> MAAVFGIQLVPKLNTSTTRRTFLPLRFDLLLDRLQSTNLHGVLYRALDFNPVDRSATVIQTYPPLNAWSPHHAFIENPLDYRDWTEFIHDRALAFVGVLTQRYPLTQNAQRYTNPLVLGAAFGDFLNARSIDIFLDRLFYDPTQDSPITAITKFPYQWTIDSNVTTDSVRTSAGCKYITLYGYDPSRPSTPATYGKHRPTYATVFYYSTLPARSRLLANLAAGPTVLEHFDSPTYGPHLLLPQTGDVLGYSSSLISQAALLMVESVMDALRDNANASASTAVTRLDQSYHPVTSFDPSTFNTLLQRATNLALLAVQGVQSESAIPAIPTMSDVRSFVARLMAEGDPQQWFPYRVDQILYWPESPFVPPIGPFYAPFRPVNFPFTTGSYTVVPDASRPLRLLPQYRNATITVQQADDAYEDTALSPLITTHGFCVTGGVFTSIYDISGDPTAYPPAQLVDAPNDYFDRERMARRDLFRRLRAPADRSAIKDRAVFDFLASLVNPTTANPVLDTSFSMAYLGASSAHANADEPVILADIRSGSIPGLPIPRRIVQFGYDVVHGSLLDLSRAVPTGTFGLVYADLDQVEDAGTDMPAANRAAIAMLGTALQMTTAGGVSVLKVNFPTRAFWTQVFNLYATHATTLHLVKPTIVNSSEVFLVFGGRQSNGALRSTTALQRALLSLYARNAAIDRAVTHIPFFGVPDDGTSDLGIDAVRLFDPMFSDAVANLPSNALASLVSRVVPSSIMFTRVPSNGPVSTTIYGKRTFLSNRRRARLRDVPMLITTTLVHQRRFTTPPTFTLFSSEAVPVTTLVAAGYNSFISEQTRNPNLAHLLDLGTGPECRILSLIPPTLQVTMSDSRPCAELMASFDPALTAYVQGDYSTAAFWNGIRCDSATAIFTIGAAAAAAGTDLIAFVQQLIPRIVAAGGTRMWLQLNTPLYEVSSLPDLIEIDLRDHVYRFNGGERVEPYADPVPLQQAIAALLPAAALSWHTLSPTCDWLPYIIGVGSPLNLSDINTAISYSRLTPILHIDTTTPPLRVNPVPTPLNQQCAIRITSLDPAAVLSVQHNGVEVIGGTPGNVISVAGAAALQYILANQEFLLQFTPTLPGIFDVFLTTLGQPPVPRGSFTITPPPTTVALNMPPPRQLDFTDVGNDARITCDPYYQLAVCIFKDGQYVRVNPEKASVVTNAPNRDLHFVLDLADNHVLLYLCDV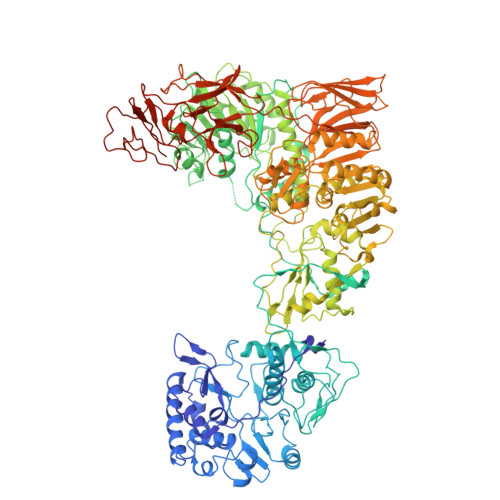TPSGLGDRIAFPIVDIYRIAFPRNTPVRASLPYTGGGAHLTSGGNPFMSLTTPPAVLPAGVALAALSTSVATQYPTYTLPAGVYEYVIE>MRIEQDFSQSLGVERLKAARLHEYNKPLRIEDVDYPRLEGRFDVIVRIAGAGVCHTDLHLVQGMWHELLQPKLPYTLGHENVGYIEEVAEGVEGLEKGDPVILHPAVTDGTCLACRAGEDMHCENLEFPGLNIDGGFAEFMRTSHRSVIKLPKDISREKLVEMAPLADAGITAYRAVKKAARTLYPGAYVAIVGVGGLGHIAVQLLKVMTPATVIALDVKEEKLKLAERLGADHVVDARRDPVKQVMELTRGRGVNVAMDFVGSQATVDYTPYLLGRMGRLIIVGYGGELRFPTIRVISSEVSFEGS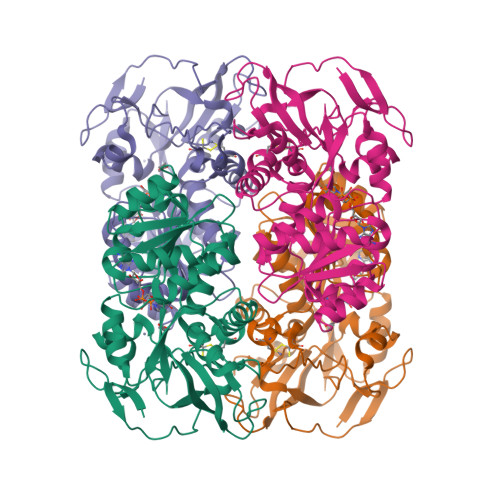LVGNYVELHELVTLALQGKVRVEVDIHKLDEINDVLERLEKGEVLGRAVLIP[2x]>MPVPNGATFPPCARKMERADGPATVLAIGTANPPNVFDQSTYPDFYFNITNSNHMTDLKTKFQRMCDKSGITKRYMYLNEEILKANPNMCAYWEKSLDVRQDMVVVEVPKLGKEAATKAIKEWGQPKSKITHVVFCTTSGVDMPGADWALTKLLGLRPSVKRLMMYQQGCFAGGTVMRVAKDLAENNKGARVLVVCSELTAVTFRGPSETHLDSLVGQALFGDGASAIIVGADPIPEVERPWFEIHYVASNILPDSDGAIDGHLREVGLTFHLMKDVPGIISKNIGTVLKDAFEK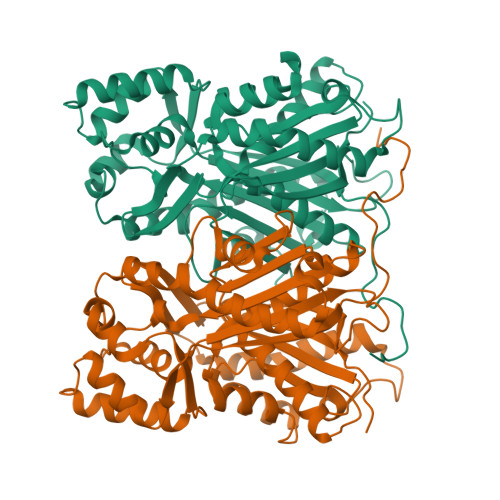VFGNEEGEVPSYNDVFWIAHPGGPAILDQVEQKLQLKTEKMAASRQVLSDYGNMSSACVLFIMDHLRKKSVEQKLATSGEGYEWGLLLGFGPGLTCETVVLRSVPLATE[4x]>SLMVSRRVQALLDQLRAQGIQDEQVLNALAAVPREKFVDEAFEQKAWDNIALPIGQGQTISQPYMVARMTELLELTPQSRVLEIGTGSGYQTAILAHLVQHV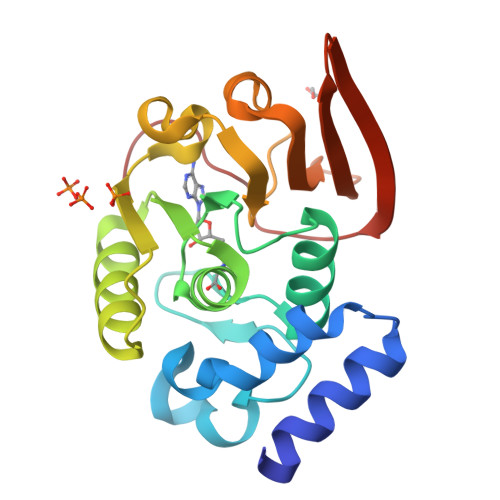CSVERIKGLQWQARRRLKNLDLHNVSTRHGDGWQGWQARAPFDAIIVTAAPPEIPTALMTQLDEGGILVLPVGEEHQYLKRVRRRGGEFIIDTVEAVRFVPLVKGELA[4x]>[2x]VANPEHYIKHPLQNRWALWFFKNDKSKTWQANLRLISKFDTVEDFWALYNHIQLSSNLMPGCDYSLFKDGIEPMWEDEKNKRGGRWLITLNKQQRRSDLDRFWLETLLCLIGESFD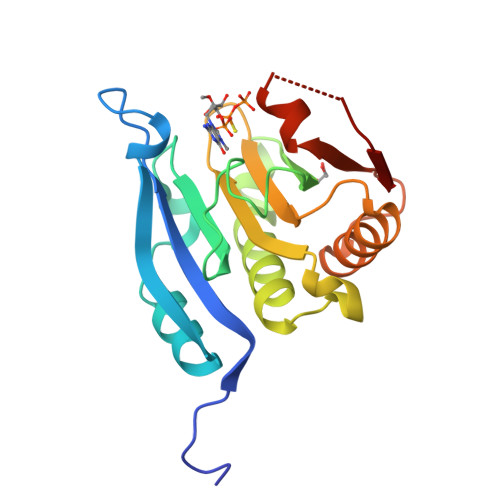DYSDDVCGAVVNVRAKGDKIAIWTTECENRDAVTHIGRVYKERLGLPPKIVIGYQSHADTATKSGSTTKNRFVV Ionotropic glutamate receptors are cation-permeable ion channels responsible for fast excitatory signal transmission in vertebrate neurons. In the α-amino-3-hydroxy-5-methyl-4-isoxazolepropionic acid receptor (AMPAR), the permeability for calcium depends exquisitely on its composition. To this aim, we investigate calcium permeation in two cation channels: The AMPA receptor GluA2 and an AMPAR channel pore mimic that incorporates the partial selectivity filter (SF) sequence of AMPAR into a bacterial NaK channel. We used the prokaryotic NaK channel as scaffold for crystallization, as in our previous study of monovalent cations.

The X-ray structures revealed distinct ion binding profiles for monovalent and divalent cations within and around the SF. The monovalent cations bind at sites S3 and S4 in the lower part of the SF formed by TTV. This is consistent with previous X-ray analysis of a NaK C-DI mutant with monovalent cations only. While monovalent cations prefer binding sites at a narrow pore, i.e., the TTV filter in NaK C-DI48 and the QQ filter in AMPAR,23 Ca2+ ions occupy more sites along the SF with substantial presence also at the wide CDI part in both NaK C-DI and AMPAR. Indeed, in NaK C-DI calcium and barium reside stably at a single site within the wide section of the selectivity filter, which shows in contrast no occupancy by monovalent ions in the presence of divalent ions.

>[4x]MWKDKEFQVLFVLTILTLISGTIFYSTVEGLRPIDALYFSVVTLTTVGCDISPQTDFGKIFTILYIFIGIGLVFGFIHKLAVNVQLPSILSNLVPR> RPATILTTQQRRAFKASFEVS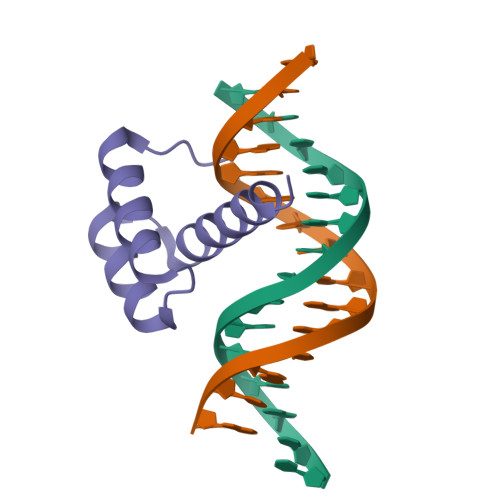SKPCRKVRETLAAETGLSVRVVQVWFQNQRAKMKKLARR> AELISK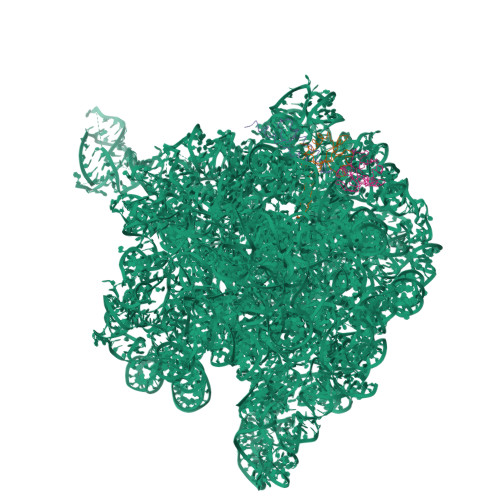EGNKVEFKVSVPAAEVNRAYDQVWAGLARDVRVPGFRPGKAPRKVIENRVGKGYVESQVRDRLLETHYSQGLRELGLNLVDATVDPQDVQSGQAFEFTVKGETYPEV;> MSHYDILQAPVISEKAYSAMERGVYSFWVSPKATKTEIKDAIQQAFGVRVIGISTMNVPGKRKRVGRFIGQRNDRKKAIVRLAEGQSIEALAGQA;> MKPSEMRNLQATDFAKEIDARKKELMELRFQAAAGQLAQPHRVRQLRREVAQLNTVKAELARKGEQQ> DQAGKSPNAVRYHGGDEIILQGFHWNVVREAPNDWYNILRQQAATIAADGFSAIWMPVPWRDFSSWSDGSKSGGGEGYFWHDFNKNGRYGSDAQLRQAASALGGAGVKVLYDVVPNHMNRGYPDKEINLPAGQGFWRNDCADPGNYPNDCDDGDRFIGGDADLNTGHPQVYGMFRDEFTNLRSQYGAGGFRFDFVRGYAPERVNSWMTDSADNSFCVGELWKGPSEYPNWD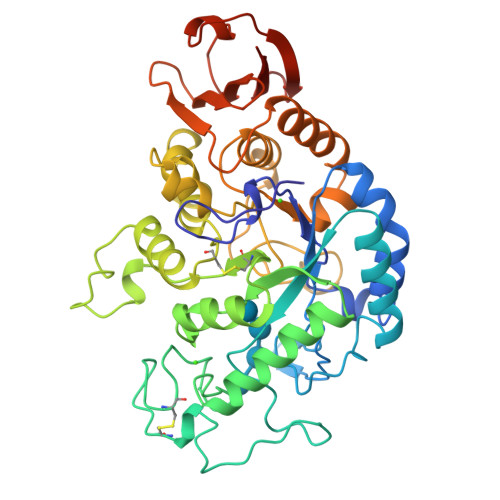WRNTASWQQIIKDWSDRAKCPVFDFALKERMQNGSIADWKHGLNGNPDPRWREVAVTFVDNHNTGYSPGQNGGQHHWALQDGLIRQAYAYILTSPGTPVVYWDHMYDWGYGDFIRQLIQVRRAAGVRADSAISFHSGYSGLVATVSGSQQTLVVALNSDLGNPGQVASGSFSEAVNASNGQVRVWRSGTGSGGGEPGA> MSEFRIHHDVNELLSLLRVHGGDGAEVYIDLLQKNRTPYVTTTVSAHSAKVKIAEFSRTPEDFLKKYDELKSKNTRNLDPLVYLLSKLTEDKETLQYLQQNAKERAELAAAAVGSSTTSINVPAAASKISMQELEELRKQLGSVATGSTLQQSLELKRKMLRDKQNKKNSGQHLPIFPAWVYERPALIGDFLIGAGISTDTALPIGTLPLASQESAVVEDLLYVLVGVDGRYVSAQPLAGRQSRTFLVDPNLDLSIRELVHRILPVAASYSAVTRFIEEKSSFEYGQVNHALAAAMRTLVKEHLILVSQLEQLHRQGLLSLQKLWFYIQPAMRTMDILASLATSVDKGECLGGSTLSLLHDRSFSYTGDSQAQELCLYLTKAASAPYFEVLEKWIYRGIIHDPYSEFMVEEHELRKERIQEDYNDKYWDQRYTIVQQQIPSFLQKMADKILSTGKYLNVVRECGHDVTCPVAKEIIYTLKERAYVEQIEKAFNYASKVLLDFLMEEKELVAHLRSIKRYFLMDQGDFFVHFMDLAEEELRKPVEDITPPRLEALLELALRMSTANTDPFKDDLKIDLMPHDLITQLLRVLAIETKQEKAMAHADPTELALSGLEAFSFDYIVKWPLSLIINRKALTRYQMLFRHMFYCKHVERQLCSVWISNKTAKQHSLHSAQWFAGAFTLRQRMLNFVQNIQYYMMFEVMEPTWHILEKNLKSASNIDDVLGHHTGFLDTCLKDCMLTNPELLKVFSKLMSVCVMFTNCMQKFTQSMKLDGELGGQTLEHSTVLGLPAGAEERARKELARKHLAEHADTVQLVSGFEATINKFDKNFSAHLLDLLARLSIYSTSDCEHGMASVISRLDFNGFYTERLERLSAERSQKATPQVPVLRGPPAPAPRVAVTAQ;>MATPDQKSPNVLLQNLCCRILGRSEADVAQQFQYAVRVIGSNFAPTVERDEFLVAEKIKKELIRQRREADAALFSELHRKLHSQGVLKNKWSILYLLLSLSEDPRRQPSKVSSYATLFAQALPRDAHSTPYYYARPQTLPLSYQDRSAQSAQSSGSVGSSGISSIGLCALSGPAPAPQSLLPGQSNQAPGVGDCLRQQLGSRLAWTLTANQPSSQATTSKGVPSAVSRNMTRSRREGDTGGTMEITEAALVRDILYVFQGIDGKNIKMNNTENCYKVEGKANLSRSLRDTAVRLSELGWLHNKIRRYTDQRSLDRSFGLVGQSFCAALHQELREYYRLLSVLHSQLQLEDDQGVNLGLESSLTLRRLLVWTYDPKIRLKTLAALVDHCQGRKGGELASAVHAYTKTGDPYMRSLVQHILSLVSHPVLSFLYRWIYDGELEDTYHEFFVASDPTVKTDRLWHDKYTLRKSMIPSFMTMDQSRKVLLIGKSINFLHQVCHDQTPTTKMIAVTKSAESPQDAADLFTDLENAFQGKIDAAYFETSKYLLDVLNKKYSLLDHMQAMRRYLLLGQGDFIRHLMDLLKPELVRPATTLYQHNLTGILETAVRATNAQFDSPEILRRLDVRLLEVSPGDTGWDVFSLDYHVDGPIATVFTRECMSHYLRVFNFLWRAKRMEYILTDIRKGHMCNAKLLRNMPEFSGVLHQCHILASEMVHFIHQMQYYITFEVLECSWDELWNKVQQAQDLDHIIAAHEVFLDTIISRCLLDSDSRALLNQLRAVFDQIIELQNAQDAIYRAALEELQRRLQFEEKKKQREIEGQWGVTAAEEEEENKRIGEFKESIPKMCSQLRILTHFYQGIVQQFLVLLTTSSDESLRFLSFRLDFNEHYKAREPRLRVSLGTRGRRSSHT[2x];>[2x]MIHELLLALSGYPGSIFTWNKRSGLQVSQDFPFLHPSETSVLNRLCRLGTDYIRFTEFIEQYTGHVQQQDHHPSQQGQGGLHGIYLRAFCTGLDSVLQPYRQALLDLEQEFLGDPHLSISHVNYFLDQFQLLFPSVMVVVEQIKSQKIHGCQILETVYKHSCGGLPPVRSALEKILAVCHGVMYKQLSAWMLHGLLLDQHEEFFIKQGPSSGNVSAQPEEDEEDLGIGGLTGKQLRELQDLRLIEEENMLAPSLKQFSLRVEILPSYIPVRVAEKILFVGESVQMFENQNVNLTRKGSILKNQEDTFAAELHRLKQQPLFSLVDFEQVVDRIRSTVAEHLWKLMVEESDLLGQLKIIKDFYLLGRGELFQAFIDTAQHMLKTPPTAVTEHDVNVAFQQSAHKVLLDDDNLLPLLHLTIEYHGKEHKADATQAREGPSRETSPREAPASGWAALGLSYKVQWPLHILFTPAVLEKYNVVFKYLLSVRRVQAELQHCWALQMQRKHLKSNQTDAIKWRLRNHMAFLVDNLQYYLQVDVLESQFSQLLHQINSTRDFESIRLAHDHFLSNLLAQSFILLKPVFHCLNEILDLCHSFCSLVSQNLGPLDERGAAQLSILVKGFSRQSSLLFKILSSVRNHQINSDLAQLLLRLDYNKYYTQAGGTLGSFGM;>[2x]MARHGPPWSRLDAQQERDVRELVRGVAGLQDEADPNFQLALNFAWSNFRFHRFLDVNSHKIEKTIEGIYEKFVIHSDLSKAASWKRLTEEFLNAPLPSIKEIKTDAHYSILSLLLCLSDSPSNSSYVETPRNKEVEKKDDFDWGKYLMEDEEMDIGPYMDTPNWSEESEEENDQQPLSREDSGIQVDRTPLEEQDQNRKLDPCISWKDEPDDRSWLEHHVVHQYWTARPSQFPHSLHLHSNLAAVWDQHLYSSDPLYVPDDRVLVTETQVIRETLWLLSGVKKLFIFQLIDGKVTVRNNIIVTHLTHSCLRSVLEQIAAYGQVVFRLQEFIDEVMGHSSESMLPGSGSVPKKSTEAPFRTYQAFMWALYKYFISFKEELAEIEKCIINNDTTITLAIVVDKLAPRLSQLKVLHKVFSTGVAEVPPDTRNVVRASHLLNTLYKAILEYDNVGEASEQTVSLLFSLWVETVRPYLQTVDEWIVHGHLWDGAREFIIQRNKNVPVNHRDFWYATYTLYSVSEKTENEEKMSDNASASSGSDQGPSSRQHTMVSFLKPVLKQIIMAGKSMQLLKNLQCAESTTCQAGARDAERKSLYTLFLESVQSRLRHGEDSTPQVLTEQQATKENLMKMQSIAESHLELDDVHDPLLAINFARMYLEQSDFHEKFAGGDVCVDRSSESVTCQTFELTLRSCLYPHIDKQYLDCCGNLMQTLKKDYRLVEYLQAMRNFFLMEGGDTMYDFYTSIFDKIREKETWQNVSFLNVQLQEAVGQRYPEDSSRLSISFENVDTAKKKLPVHILDGLTLSYKVPWPVDIVISLECQKIYNQVFLLLLQIKWAKYSLDVLLFGELVSTAEKPRLKEGLIHEQDTVAQFGPQKEPVRQQIHRMFLLRVKLMHFVNSLHNYIMTRILHSTGLEFQHQVEEAKDLDQLIKIHYRYLSTIHDRCLLREKVSFVKEAIMKVLNLALMFADGWQAGLGTWRMESIEKMESDFKNCHMFLVTILNKAVCRGSFPHLESLALSLMAGMEQS;> MASITQLFDDLCEALLPAAKTHLGQRSVNRKRAKRSLKKVAYNALFTNLFQDETQQLQPDMSKLPARNKILMLSFDLRVGGLGPKADRLEELVEELEAAPCCPLLEVGSVLDLLVQLAGSGPPQVLPRKRDYFLNNKHVGRNVPYSGYDCDDLSVFEMDVQSLISREECLCHSMIQETLQVMEAAPGTGLPTVGLFSFGDPCGDRFERDTRVSLFGALVHSRTYDMDVRLGLPPVPDNADLSGLAIKVPPSVDQWEDEGFQSASNLTPDSQSEPSVTPDVDLWEAALTYEASKRRCWERVGCPPGHREEPYLTEAGRDAFDKFCRLHQGELQLLAGGVLQAPQPVLVKECELVKDVLNVLIGVVSATFSLCQPAQAFVVKRGVHVSGASPESISSLLSEVAEYGTCYTRLSHFSLQPVLDSLYSKGLVFQAFTSGLRRYLQYYRACVLSTPPTLSLLTIGFLFKKLGRQLRYLAELCGVGAVLPGTCGGGPRAAFPTGVKLLSYLYQEALHNCSNEHYPVLLSLLKTSCEPYTRFIHDWVYSGVFRDAYGEFMIQVNHEYLSFRDKLYWTHGYVLISKEVEDCVPVFLKHIAHDIYVCGKTINLLKLCCPRHYLCWSDVPVPRISVIFSLEELKEIEKDCAVYVGRMERVARHSSVSKEEKELRMEIAKQELIAHAREAASRVLSALSDRQMSERMALDARKREQFQRLKEQFVKDQERRQAARQEELDDDFSYARELRDRERRLKSLEEELERKARQALVDHYSKLSAEAARREQKALWRIQRHRLESARLRFLLEDEKHIQEMLKAVSEAHQPQEPPDVLLSVHPQVTSPGPEHPEGGQGCDSGSAEQHSPAWDGWNRPGLLTPQPLKPLAVGAGGRGLQQAEGARPFSDSLSIGDFLPVGPGAEPSVQTGMVPLLEVALQTINLDLPPSAPGEAPAAASTQPSRPQEYDFSTVLRPAVATSPAPGPLQAAECSLGSSGLQLWEDSCGKMDACGSASRETLLPSHPPRRAALEEGSSQPTERLFGQVSGGGLPTGDYASEIAPTRPRWNTHGHVSDASIRVGENVSDVAPTQPRWNTHGHVSNASISLGESVSDVAPTRPRWNIHGHVSNASIRVGENVSDVAPTRPRWNTHGHVSNASIRVGENVSDVAPTRPRWNTHGHVSDASISLGESVSDMAPARPRWNTHGHVSDASISLGESVSDMAPTRPRWNTHGHVSDTSIRVGENVSDVAPIRSRCNTHGHVSDASISLGEPVSDVVSTRPRWNTHVPIPPPHMVLGALSPEAEPNTPRPQQSPPGHTSQSALSLGAQSTVLDCGPRLPVEVGPSLSSPSSGCGEGSISVGENVSDVAPTQPWWPNTPGDSVSEELGPGRSGDTEDLSPNWPLNSQEDTAAQSSPGRGEEAEASAAEAQGGEQAYLAGLAGQYHLERYPDSYESMSEPPIAHLLRPVLPRAFAFPVDPQVQSAADETAVQLSELLTLPVLMKRSITAPLAAHISLVNKAAVDYFFVELHLEAHYEALRHFLLMEDGEFAQSLSDLLFEKLGAGQTPGELLNPLVLNSVLSKALQCSLHGDTPHASNLSLALKYLPEVFAPNAPDVLSCLELRYKVDWPLNIVITEGCVSKYSGVFSFLLQLKLMMWALKDVCFHLKRTALLSHMAGSVQFRQLQLFKHEMQHFVKVIQGYIANQILHVTWCEFRARLATVGDLEEIQRAHAEYLHKAVFRGLLTEKAAPVMNVIHSIFSLVLKFRSQLISQAWGPPGGPRGAEHPNFALMQQSYNTFKYYSHFLFKVVTKLVNRGYQPHLEDFLLRINFNNYYQDA;>[6x]MPREIITLQLGQCGNQIGFEFWKQLCAEHGISPEGIVEEFATEGTDRKDVFFYQADDEHYIPRAVLLDLEPRVIHSILNSPYAKLYNPENIYLSEHGGGAGNNWASGFSQGEKIHEDIFDIIDREADGSDSLEGFVLCHSIAGGTGSGLGSYLLERLNDRYPKKLVQTYSVFPNQDEMSDVVVQPYNSLLTLKRLTQNADCVVVLDNTALNRIATDRLHIQNPSFSQINQLVSTIMSASTTTLRYPGYMNNDLIGLIASLIPTPRLHFLMTGYTPLTTDQSVASVRKTTVLDVMRRLLQPKNVMVSTGRDRQTNHCYIAILNIIQGEVDPTQVHKSLQRIRERKLANFIPWGPASIQVALSRKSPYLPSAHRVSGLMMANHTSISSLFERTCRQYDKLRKREAFLEQFRKEDMFKDNFDEMDTSREIVQQLIDEYHAATRPDYISWGTQEQ;>MASSSGAGAAAAAAAANLNAVRETMDVLLEISRILNTGLDMETLSICVRLCEQGINPEALSSVIKELRKATEALKAAENMTS[2x]

The gamma-tubulin ring complex (γ-TuRC) is the principal microtubule nucleation template in vertebrates. Microtubules are formed de novo in a process termed nucleation, which is spatially and temporally highly controlled by γ-tubulin complexes, composed of γ-tubulin1 and associated γ-tubulin-complex proteins (GCP). In most eukaryotes, microtubules are templated from a preassembled γ-tubulin ring complex (γ-TuRC) that determines the position and direction of microtubule growth. Here, we used cryo-EM to identify and characterize γ-TuRC assembly intermediates after recombinant expression of the complex, which allowed us to delineate a comprehensive stepwise assembly pathway from a stable 6-spoked core to the mature 14-spoked γ-TuRC, identifying successive stabilization and conformational locking of γ-TuSC units as central principles in the assembly process.

Extensive 3D classification revealed a core of six γ-tubulin-GCP spokes as the minimal stable and most abundant entity in this experiment. This 6-spoke assembly intermediate was resolved to 5.3 Å resolution, sufficient to unambiguously determine the identity and sequential arrangement of spokes based on secondary structure features of the GCP proteins. The cryo-EM density of the 6-spoke intermediate revealed that the first module of the lumenal bridge has already been formed by recruitment of the MZT1-GCP3 module to the GCP3(8) GRIP1 domain. Since only one copy of GCP3 is present in this intermediate, this clearly indicates that the MZT1-GCP3 module of GCP3(8) (rather than any other copy of GCP3) is involved in forming the lumenal bridge. Surprisingly, the outer surface of the GCP3(8) GRIP2 domain is associated with an additional MZT1-containing module. As the only MZT1-GCP3 module present in the 6-spoke intermediate was already stably recruited into the lumenal bridge, MZT1-GCP5 and MZT1-GCP6 were the only other candidates to represent this additional MZT1 module. Notably, GCP3(8) and the adjacent GCP4(9) subunit create a structurally unique binding site for this MZT1-GCP5 module, which likely explains the specific binding of MZT1-GCP5 to the outer surface of GCP3(8), while MZT1-GCP3(8) remains available to form the first module of the lumenal bridge. The overall stabilizing role of the GCP6 GRIP1-NTE is further supported by direct contacts of GCP6 with the GCP5(10) GRIP1-NTE and the GRIP1 domains of GCP4(9), GCP5(10), and GCP4(11), effectively bridging all GCP subunits of the intermediate. Taken together, we conclude that the GCP6 GRIP1-NTE plays a central role in the formation of the stable 6-spoke intermediate, providing a structure-based rationale for the effects of GCP6 truncations on γ-TuRC assembly previously observed in sucrose gradient sedimentation experiments.>[2x]SNASVTFSYLAETDYPVFTLGGSTADAARRLAASGCACAPVLDGERYLG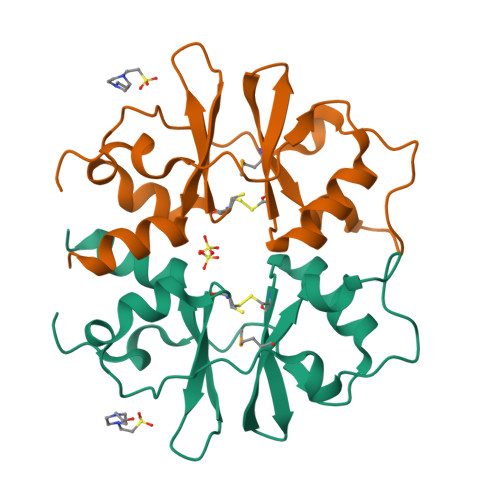MVHLSRLLEGRKGWPTVKEKLGEELLETVRSYRPGEQLFDNLISVAAAKCSVVPLADEDGRYEGVVSRKRILGFLAERI> MQSVGGDSSADRLFPPQWICCDIRYLDVSILGKFAVVMADPPWDIHMELPYGTLTDDEMRRLNIPVLQDDGFLFLWVTGRAMELGRECLNLWGYERVDEIIWVKTNQLQRIIRTGRTGHWLNHGKEHCLVGVKGNPQGFNQGLDCDVIVAEVRSTSHKPDEIYGMIERLSPGTRKIELFGRPHNVQPNWITLGNQLDGIHLLDPDVVARFKQRYPDGIISKPKNL;> GSGQSLNPHNDYCQHFVDTGHRPQNFIRDVGLADRFEEYPKLRELIRLKDELIAKSNTPPMYLQADIEAFDIRELTPKFDVILLEPPLEEYYRETGITANEKCWTWDDIMKLEIDEIAAPRSFIFLWCGSGEGLDLGRVCLRKWGYRRCEDICWIKTNKNNPGKTKTLDPKAVFQRTKEHCLMGIKGTVKCSTDGDFIHANVDIDLIITEEPEIGNIEKPVEIFHIIEHFCLGRRRLHLFGRDSTIRPGWLTVGPTLTNSNYNAETYASYFSAPNSYLTGCTEEIERLRPKSPPPKSKSDRGGGAPRGGGRGGTSAGRGRE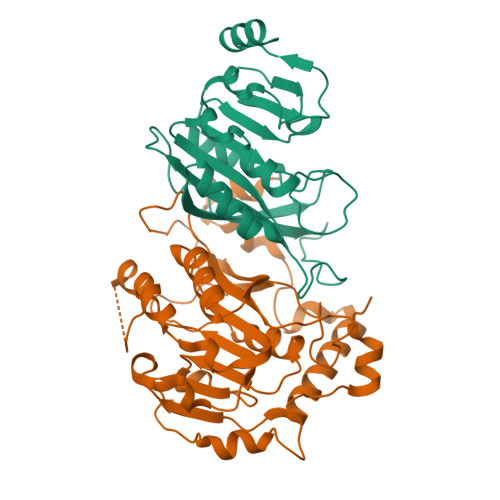RNRSNFRGERGGFRGGRGGAHRGGFPPR> HGSPVDICTA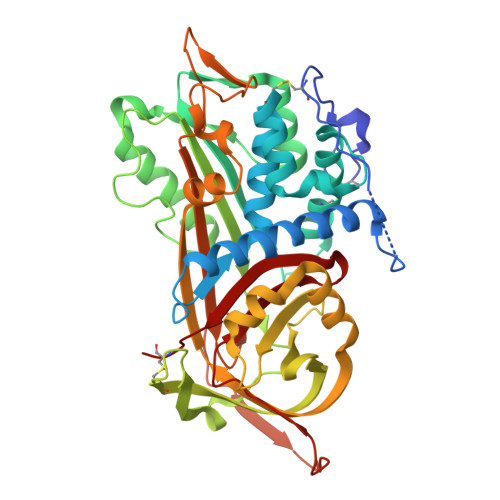KPRDIPMNPMCIYRSPEKKATEDEGSEQKIPEATNRRVWELSKANSRFATTFYQHLADSKNDNDNIFLSPLSISTAFAMTKLGACNDTLQQLMEVFKFDTISEKTSDQIHFFFAKLNCRLYRKANKASKLVSANRLFGDKSLTFNETYQDISELVYGAKLQPLDFKENAEQSRAAINKWVSNKTEGRITDVIPSEAINELTVLVLVNTIYFKGLWKSKFSPENTRKELFYKADGESCSASMMYQEGKFRYRRVAEGTQVLELPFKGDDITMVLILPKPEKSLAKVEKELTPEVLQEWLDELEEMMLVVHMPRFRIEDGFSLKEQLQDMGLVDLFSPEKSKLPGIVAEGRDDLYVSDAFHKAFLEVNEEGSAAAASTAVVIAGRSLNPNRVTFKANRPFLVFIREVPLNTIIFMGRVANPCVK> MQNITQSWFVQGMIKATTDAWLKGWDERNGGNLTLRLDDADIAPYHDNFHQQPRYIPLSQPMPLLANTPFIVTGSGKFFRNVQLDPAANLGIVKVDSDGAGYHILWGLTNEAVP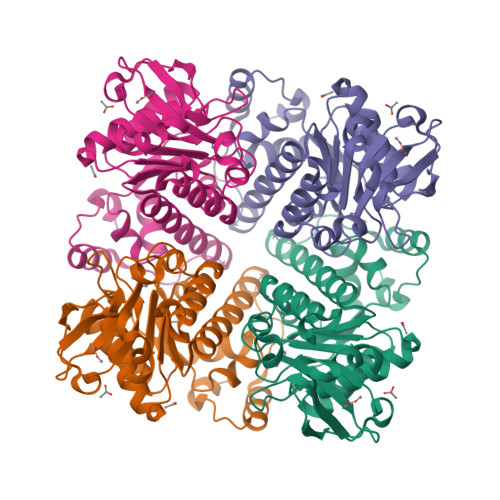TSELPAHFLSHCERIKATNGKDRVIMHCHATNLIALTYVLENDTAVFTRQLWEGSTECLVVFPDGVGILPWMVPGTDAIGQATAQEMQKHSLVLWPFHGVFGSGPTLDETFGLIDTAEKSAQVLVKVYSMGGMWQTISREELIALGKRFGVTPLASALSL> MLPPGKPEIFKCRSPNKETFTCWWRPGTDGGLPTNYSLTYHREGETLMHECPDYITGGPNSCHFGKQYTSMWRTYIMMVNATNQMGSSFSDELYV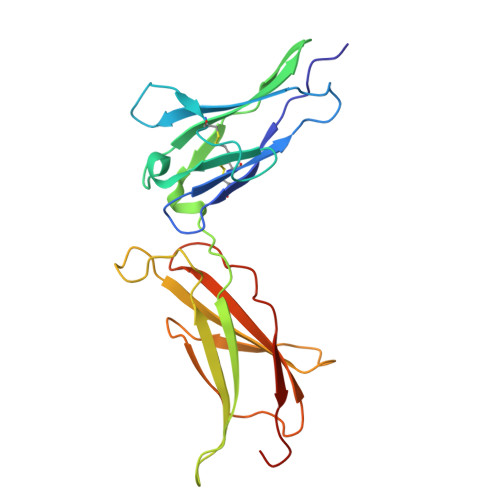DVTYIVQPDPPLELAVEVKQPEDRKPYLWIKWSPPTLIDLKTGWFTLLYEIRLKPEKAAEWEIHFAGQQTEFKILSLHPGQKYLVQVRCKPDAGYWSAWSPATFIQIPSDFTMND>MAHHHHHHMKSKLTVVYYDLESNIAEEILSGNIMPDGNFLIQEIPLFAPNLALNDIVAIEREDKMLFFDHLIKASGNTTINIVVLDHFPKDLLAAIEEHSGKIRKNGENYLSVNFPPKKY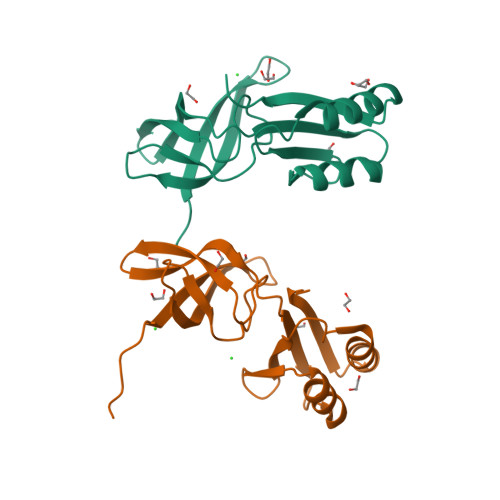NSDLKGILNRYEEANILSYREACLGFS[2x]> SRHSEKIAIRDFQVGDLVLIILDERHDNYVLFTVSPTLYFLHSESLPALDLKPG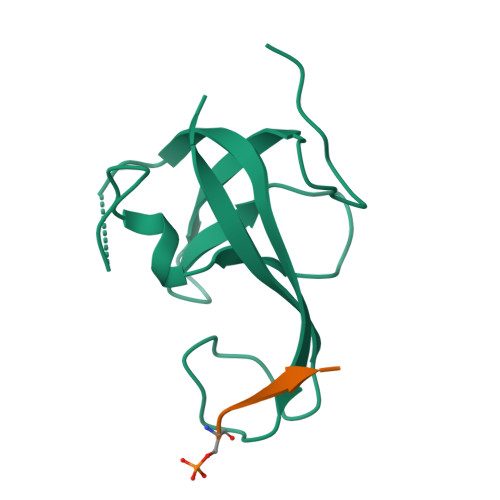EGASGASRRPWVLGKVMEKEYCQAKKAQNRFKVPLGTKFYRVKAVSWNKKV;> GTSSEFEVVTPEE METHYL N-[(2S,3R)-3-AMINO-2-HYDROXYHEPTANOYL]-L-SERYL-L-LEUCINATE 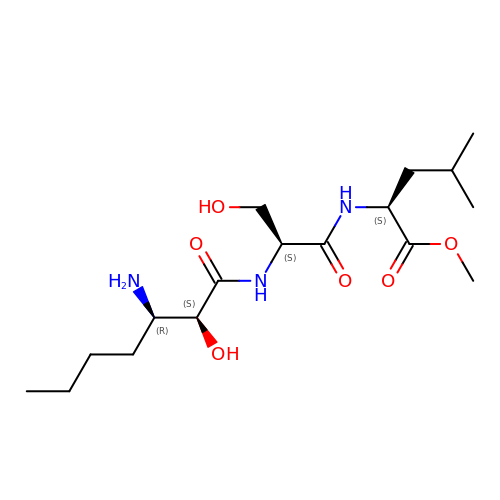| C17 H33 N3 O6 | ZERLQNOHSLWIIV-RFGFWPKPSA-N>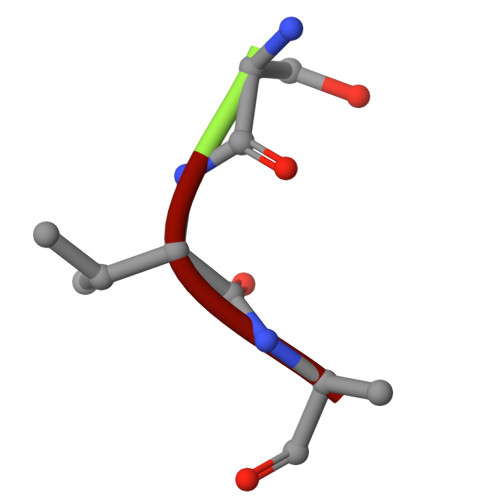 SVA> MHHHHHHGSGEGQGPKKQTRLGLEAKKEENLADWYSQVITKSEMIEYHDISGCYILRPWAYAIWEAIKDFFDAEIKKLGVENCYFPMFVSQSALEKEKTHVADFAPEVAWVTRSGKTELAEPIAIRPTSETVMYPAYAKWVQSHRDLPIKLNQWCNVVRWEFKHPQPFLRTREFLWQEGHSAFATMEEAAEEVLQILDLYAQVYEELLAIPVVKGRKTEKEKFAGGDYTTTIEAFISASGRAIQGGTSHHLGQNFSKMFEIVFEDPKIPGEKQFAYQNSWGLTTRTIGVMTMVHGDNMGLVLPPRVACVQVVIIPCGITNALSEEDKEALIAKCNDYRRRLLSVNIRVRADLRDNYSPGWKFNHW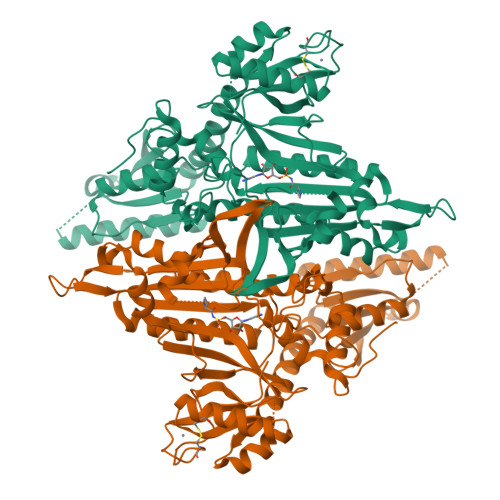ELKGVPIRLEVGPRDMKSCQFVAVRRDTGEKLTVAENEAETKLQAILEDIQVTLFTRASEDLKTHMVVANTMEDFQKILDSGKIVQIPFCGEIDCEDWIKKTTARDQDLEPGAPSMGAKSLCIPFKPLCELQPGAKCVCGKNPAKYYTLFGRSY>[2x]SLANIREIAKRAGISIATVSRHLNNTGYVSEDAREKIQKVVDELNYTPNALARAMFTKNSKTIGLMVPNISNPFFNQMASVIEEYAKNKGYTLFLCNTDDDKEKEKTYLEVLQSHRVAGIIASRSQCEDEYANI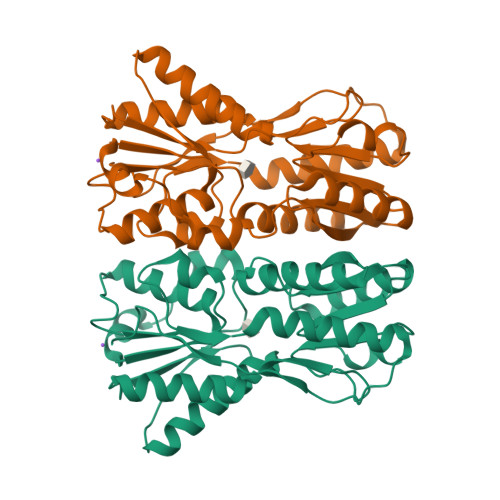DIPVVAFENHILDNIITISSDNYNGGRMAFDHLYEKGCRKILHIKGPEVFEATELRYKGFLDGARAKDLEIDFIEFQHDFQVKMLEEDINSMKDIVNYDGIFVFNDIAAATVMRALKKRGVSIPQEVQIIGFDNSFIGELLYPSLTTINQPIEALAYTIIELLIKIINGEGVLIEDYIMEVKLIERETTISLKDEG>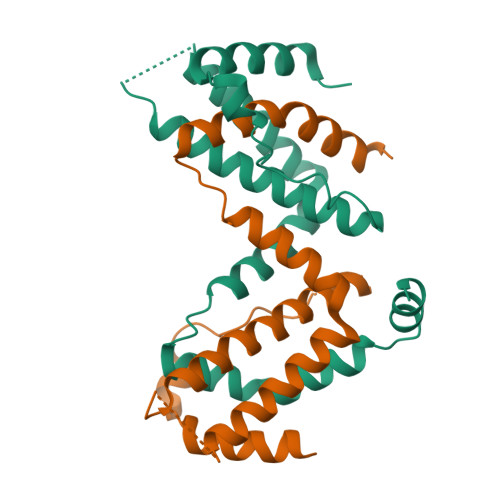[2x]SHIPARMNKTIQNLLQHYNISNKDRFNGKPVFPKEPLSGRMETKMLFMGGVLETYEKLIGQMLEQLPNTTPPTAGSREGLNSAAPEVSVRTDLNYILKKVQELRTNRFKEQSKLLQGLHDLGDIKMNNFIIQSKALWELQWMYEEASSLSNNTKMQRRRRRRRRQARKVKTPTRA(3S,5R)-5-[(2R,3R)-1,3-dihydroxybutan-2-yl]-3-({(3R)-1-[(1E)-ethanimidoyl]pyrrolidin-3-yl}sulfanyl)-L-proline 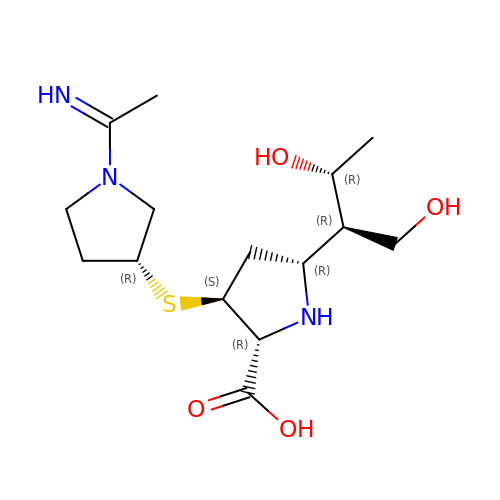| C15 H27 N3 O4 S | BSDSVSWWQWOWPI-SXFXLBHASA-N> DNNFYSVEIGDSTFTVLKRYQNLKPIGSGAQGIVCAAYDAILERNVAIKKLSRPFQNQTHAKRAYRELVLMKCVNHKNIIGLLNVFTPQKSLEEFQDVYIVMELMDANLCQVIQMELDHERMSYLLYQMLCGIKHLHSAGIIHRDLKPSNIVVKSDCTLKILDFGLARTAGTSFMMTPYVVTRYYRAPEVILGMGYKENVDLWSVGCIMGEMVCHKILFPGRDYIDQWNKVIEQLGTPCPEFMKKLQPTVRTYVENRPKYAGYSFEKLFPDVLFPADSEHNKLKASQARDLLSKMLVIDASKRISVDEAL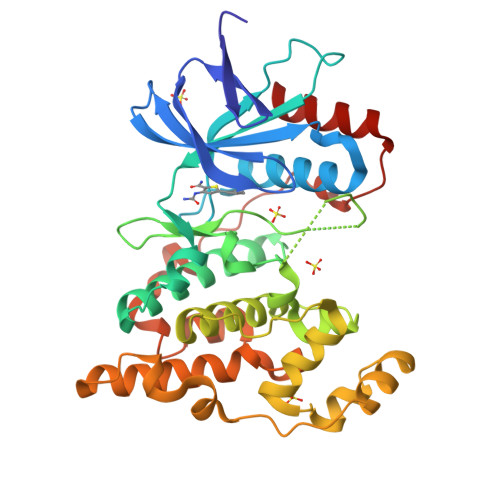QHPYINVWYDPSEAEAPPPKIPDKQLDEREHTIEEWKELIYKEVMDLE>GSHMAIVLGRNQYGKAEVRVFRVYRDTPRHEVRDLNVWTALRGDFTDAHVTGDQSHVLPTDTQKNTVYALAKKEGIRAIEDFALTLGDHFLRQVPAATGARIAIEEYAWDRIDVDGTGHDHGFVRRGQGTR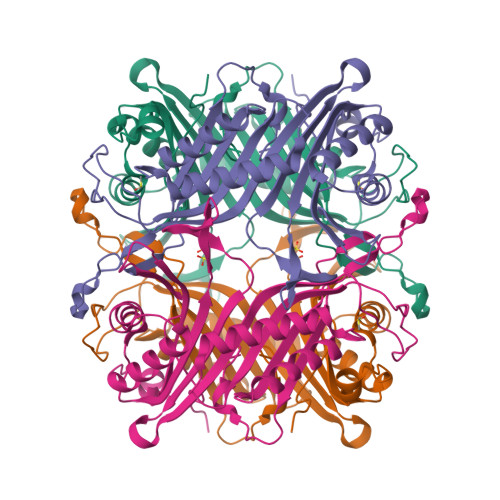TTVVTVEGRGDERRAWVLSGISDLIIAKTTGSEFHGFLKDEYTTLEETHDRILATSLHTRWRYLTTDVDWDKTFASVRSILLRQFATVHSLALQQTLYAMGSAVLEAHPEIAEIRLSAPNKHHFLVDLQPFGLDNPGEVFYASDRPYGLIEASVVRDDVPEAPEAWLATPGFC[2x]> GEIEFIESSKDAGFPVINTPSKTKLEPSVFHQVFEGNKEPAVLRSGDPRLKANFEEAIFSKYIGNVNTHVDEYMLEAVDHYAGQLATLDISTEPMKLEDAVYGTEGLEALDLTTSAGYPYVALGIKKRDILSKKTKDLTKLKECMDKYGLNLPMVTYVKDE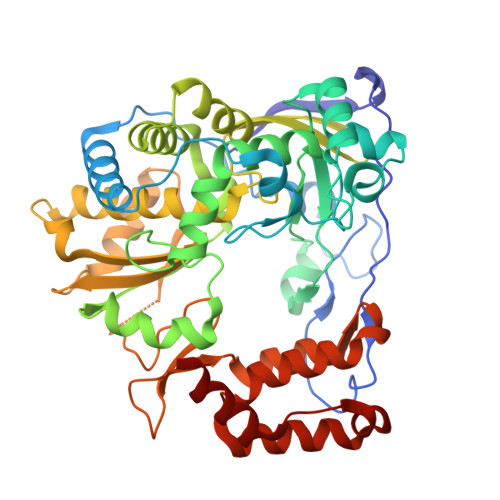LRSIEKVAKGKSRLIEASSLNDSVAMRQTFGNLYKTFHLNPGVVTGSAVGCDPDLFWSKIPVMLDGHLIAFDYSGYDASLSPVWFACLKMILEKLGYTHKETNYIDYLCNSHHLYRDKHYFVRGGMPSGCSGTSIFNSMINNIIIRTLMLKVYKGIDLDQFRMIAYGDDVIASYPWPIDASLLAEAGKGYGLIMTPADKGECVNEVTWTNVTFLKRYFRADEQYPFLVHPVMPMKDIHESIRWTKDPKNTQDHVRSLCLLAWHNGEHEYEEFIRKIRSVPVGRCLTLPAFSTLRRKWLDSF> MGKVIRSLNRFGKKVGNALTSNTAKKIYSTIGKAAERFAESEIGSAAIDGLVQGSVHSIITGESYGESVKQAVLLNVLGSGEEIPDPLSPGERGIQAKLKELEDEQRNELVRLKYNDKIKEKFGKELEEVYNFMNGEANAEIEDEKQFDILNKAVTSYNKILTEEDLQMRRLATALQKEIGERTHAETVMVKEYRDKIDALKNAIEVERDGMQEEAIQEIAGMTADVLEAASEEVPLIGAGMATAVATGRAIEGAYKLKKVINALSGIDLTHLRTPKIEPSVVSTILEYRAKEIPDNALAVSVLSKNRAIQENHKELMHIKNEILPRFKKAMDEEKEICGIEDKVIHPKVMMKFKIPRAQQPQIHVYSAPWDSDDVFFFHCISHHHANESFFLGFDLSIDLVHYEDLTAHWHALGAAQTAAGRTLTEAYREFLNLAISNAFGTQMHTRRLVRSKTVHPIYLGSLHYDISFSDLRGNAQRIVYDDELQMHILRGPIHFQRRAILGALKFGCKVLG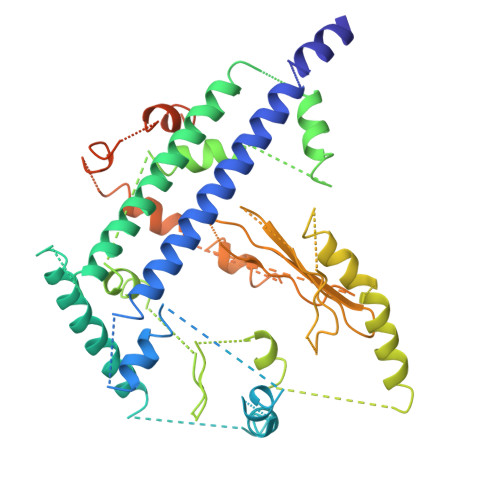DRLDVPLFLRNA> SDILFP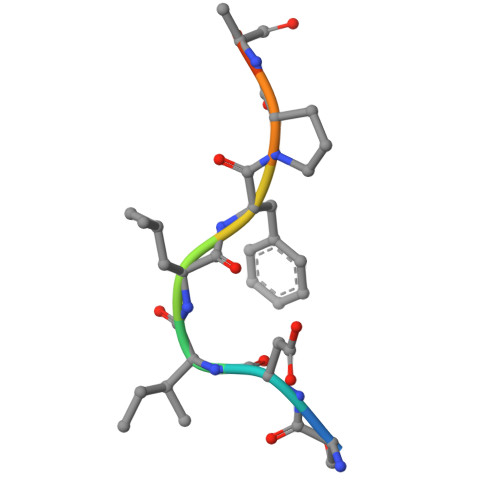ADS4-[(2-{4-[(PHENYLCARBAMOYL)AMINO]-1H-PYRAZOL-3-YL}-1H-BENZIMIDAZOL-5-YL)METHYL]MORPHOLIN-4-IUM 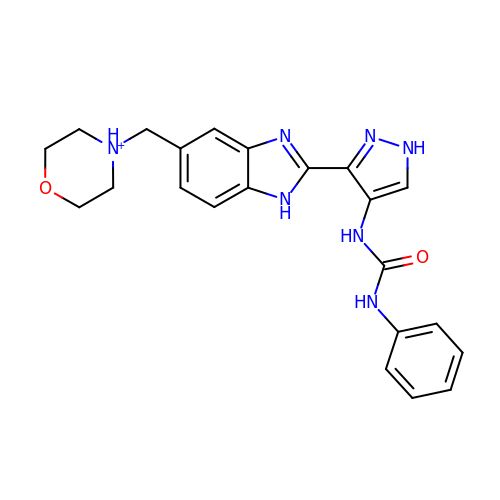| C22 H24 N7 O2 | SOTHNRIRXPUQEZ-UHFFFAOYSA-O>[8x]MTVQAQNIDAITAGAMPHEEPELTDGFHLVIDALKLNGIETIYNVPGIPITDLGRLAQAEGLRVISFRHEQNAGNAAAIAGFLTKKPGICLTVSAPGFLNGLTALANATTNCFPMILISGSSEREIVDLQQGDYEEMDQLAIAKPLCKAAFRVLHAADIGIGVARAIRAAVSGRPGGVYLDLPAKLFSQVIDADLGARSLVKVIDAAPAQLPAPAAIARALDVLKSAERPLIILGKGAAYAQADEAVRALVEESGIPYVPMSMA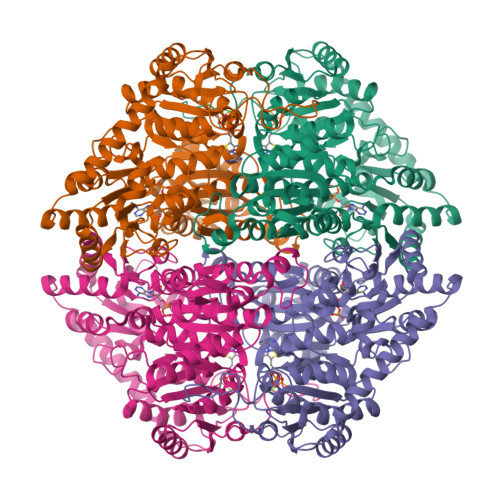KGLLPDTHPLSAGAARSTALKDSDVVLLVGARLNWLLSHGKGKTWGEPGSKRFIQIDIEPREMDSNVEIVAPVVGDIGSCVEALLDGIRKDWKGAPSNWLETLRGKREANIAKMAPKLMKNSSPMCFHSALGALRTVIKERPDAILVNEGANTLDLARGIIDMYQPRKRLDVGTWGVMGIGMGFAVAAAVETGKPVLAVEGDSAFGFSGMEVETICRYELPVCIVIFNNNGIYRGTDTDPTGRDPGTTVFVKNSRYDKMMEAFGGVGVNVTTPDELKRAVDEAMNSGKPTLINAEIDPAAGSESGNIGSLNPQSTLKKK3-[5-methylsulfanyl-4-(3,4,5-trimethylphenyl)-1,2,4-triazol-3-yl]propan-1-ol 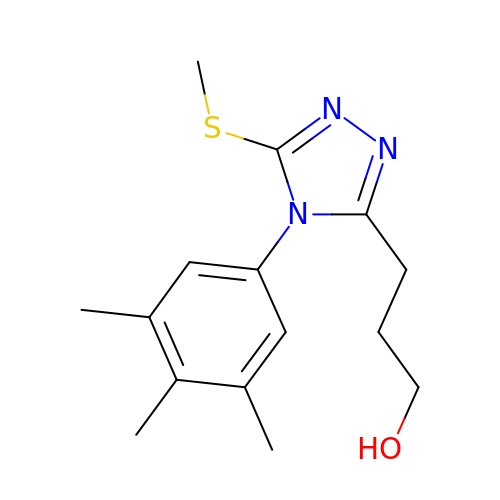| C15 H21 N3 O S | WLYAKMVSMAFGQO-UHFFFAOYSA-N> MTKALFFDIDGTLVSFETHRIPSSTIEALEAAHAKGLKIFIATGRPKAIINNLSELQDRNLIDGYITMNGAYCFVGEEVIYKSAIPQEEVKAMAAFCEKKGVPCIFVEEHNISVCQPNEMVKKIFYDFLHVNVIPTVSFEEASNKEVIQMTPFITEEEEKEVLPSIPTCEIGRWYPAFADVTAKGDTKQKGIDEIIRHFGIKLEETMSFGDGGNDISMLRHAAIGVAMGQAKEDVKAAADYVTA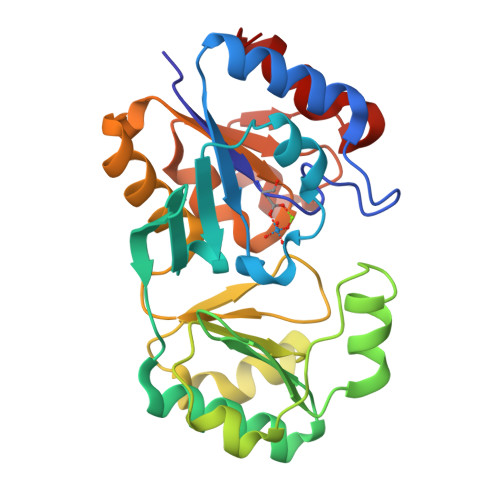PIDEDGISKAMKHFGII> MPSAHSVKLRPLEREDLRYVHQLDNNASVMRYWFEEPYEAFVELSDLYDKHIHDQSERRFVVECDGEKAGLVELVEINHVHRRAEFQIIISPEYQGKGLATRAAKLAM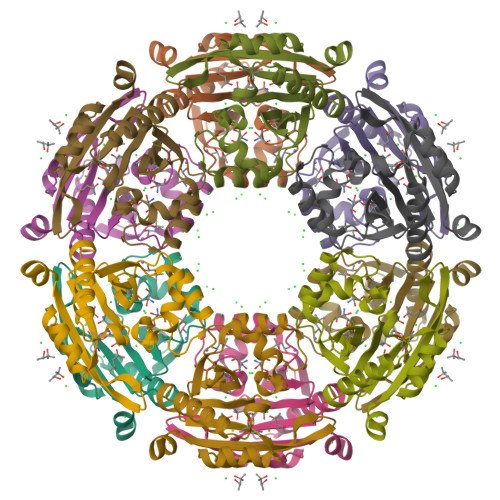DYGFTVLNLYKLYLIVDKENEKAIHIYRKLGFSVEGELMHEFFINGQYRNAIRMCIFQHQYLAEHKTPGQTLLKPTAQ> DYDYGTDTCPFPVLANKTNKAKFVGCHQKCN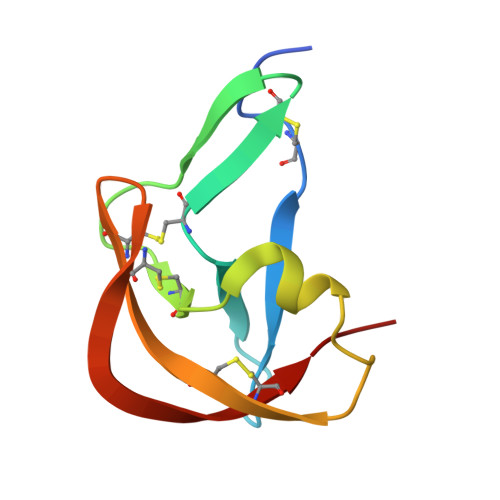GGDQKLTDGTACYVVERKVWDRMTPMLWYECPLGECKNGVCEDLRKKEDCRKGN>MSKNRSSLQSGPLNSELLEEQKQEIYEAFSLFDMNNDGFLDYHELKVAMKALGFELPKREILDLIDEYDSEGRHLMKYDDFYIVMGEKILKRDPLDEIKRAFQLFDDDHTGKISIKNLRRVAKELGETLTDEELRAMIEEFDLDGDGEINENEFIAICT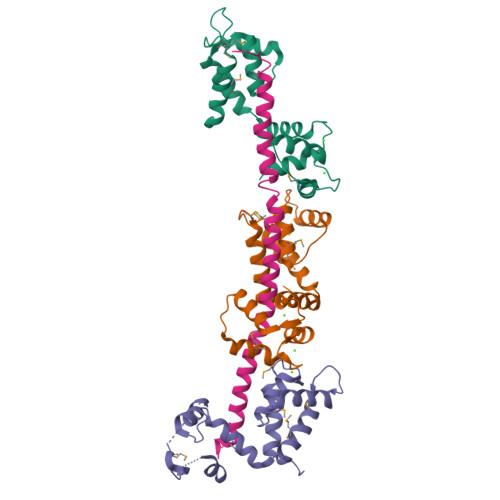DS[3x];> GPLGSNEEANRFANQAKLRVQEAVFYIWSDKTLKYSQMANDEAESFRNTWLLFRSFQQWITLTQTFKEQSRLADQAFLNKMFRKILKAQEHWKH>MSERRDAILKASATAIAQRGIRGLRVNDVAEVAGVSPGLLYYHFKDRIGLLEAALNYINDRARAYRSEGEGSGDSARDRLTRSLLGEIQDRPEVVENSLAWNELRASAVYEEALRDPLARTTAAWVSEIADAIVQAQATGEISRSLDPQPTAVTMTALVEGLSGRWLCKEIST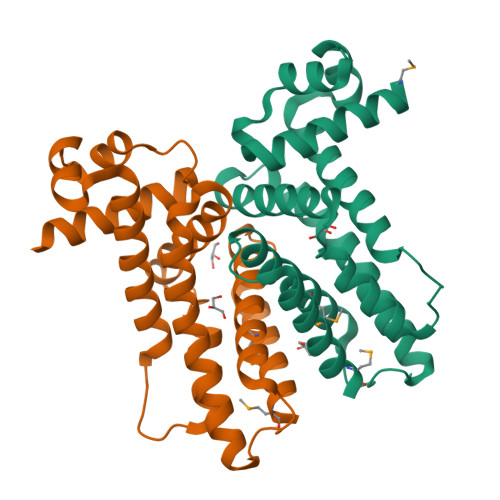EDARSHLLGAIDVVMSEPTHHTADTPVTPTPKEYR[2x]>MTTSESPDAYTESFGAHTIVKPAGPPRVGQPSWNPQRASSMPVNRYRPFAEEVEPIRLRNRTWPDRVIDRAPLWCAVDLRDGNQALIDPMSPARKRRMFDLLVRMGYKEIEVGFPSASQTDFDFVREIIEQGAIPDDVTIQVLTQCRPELIERTFQACSGAPRAIVHFYNSTSILQRRVVFRANRAEVQAIATDGARKCVEQAAKYPGTQWRFEYSPESYTGTELEYAKQVCDAVGEVIAPTPERPIIFNLPATVEMTTPNVYADSIEWMSRNLANRESVILSLHPHNDRGTAVAAAELGFAAGADRIEGCLFGNGERTGNVCLVTLGLNLFSRGVDPQIDFSNIDEIRRTVEYCNQLPVHERHPYGGDLVYTAFSGSHQDAINKGLDAMKLDADAADCDVDDMLWQVPYLPIDPRDVGRTYEAVIRVNSQSGKGGVAYIMKTDHGLSLPRRLQIEFSQVIQKIAEGTAGEGGEVSPKEMWDAFAEEYLAPVRPLERIRQHVDAADDDGGTTSITATVKINGVETEISGSGNGPLAAFVHALADVGFDVAVLDYYEHAMSAGDDAQAAAYVEASVTIASPAQPGEAGRHASDPVTIASPAQPGEAGRHASDPVTSKTVWGVGIAPSITTASLRAVVSAVNRAAR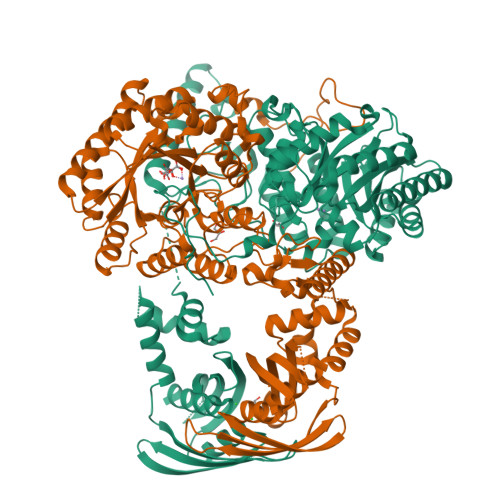[2x]> HANEQIIDMPENSEMKSMKND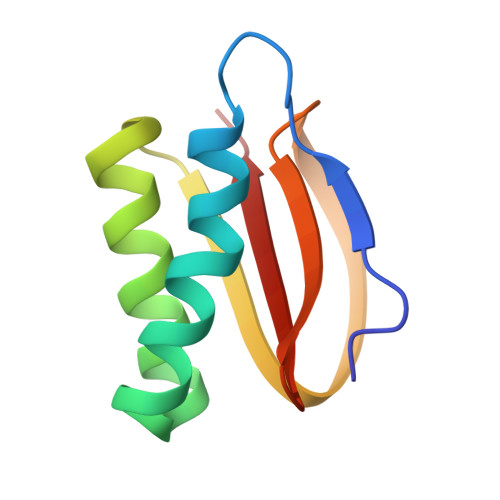AFSQAKFAVENYKFENKISSHIKKFFDEKYGPNWHCVVGKHFNAYVSYDSKNFIFFYEGQLAILLYRKG>[9x]MADISRSEVATLIQEAYANDLLASAKKGSTVLQAFPTVNMGTKTTHLPVLATLPGASWVSESATEPEGVKPTSEATWADRTLVAEEVAVIIPVHENVVDDASTSLLEEIAALGGQAIGKKLDQAVIFGTDKPSSWVSPALLPAAVAANQDYTI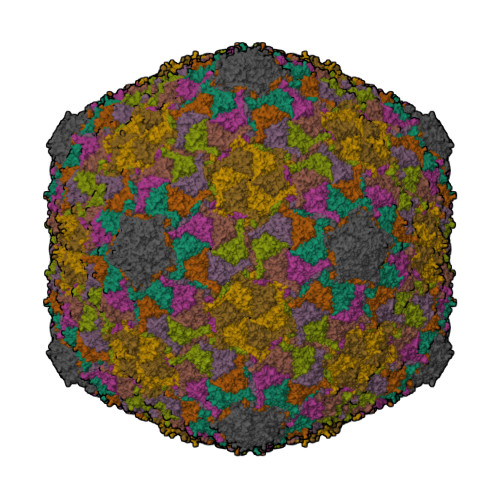VPGDANEDDLIGCINRASKAVAAAGYMPDTLLASLGFRFDVANLRDANGNPIFRDESFNGFGTYFNANGAWPVGVAEALVVDSSRVRIGVRQDITVKFLDQATVGSINLAERDMIALRLKARFAYVLGNGATAVGDNKTPVGAVVPDGS>[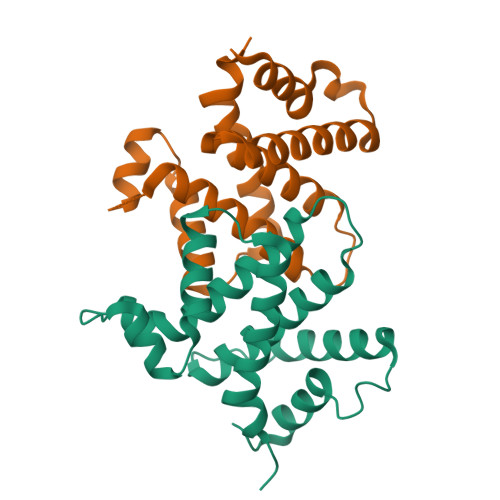3x]MPWKSSDEVVYLKGLFFPADREQISRDELYRQYEEAISLVEMYSSRTRVSHILQSTAHLFSALMMLESFEGGLDDTVRLTASMTIIRFVNGLLDPNQQSQFAIPLHLLAKKIDLPSLFVEFRHSATHDALPSLEMCKTCVDRAIDWVWDHYWDGVLSI>GAMGSDEQPHIGNYRLLKTLGKGNFAKVKRARHILTGREVAIKIIDKTQLNPTSLQKLFREVRIMKILNHPNIIKLFEVIETEKTLYLIMEYASKGEVYDYLVEHGRMKEKEARSKFRQIVSAVQYCHQKRIVHRDLKAENLLLDADMNIKIADFGFSNEFTVGGKLDTFCGSPPYAAPELFQGKKYDGPEVDVWSLGVILYTLVSGSLPFDGQNLKELRERVLRGKYRIPFYMSTD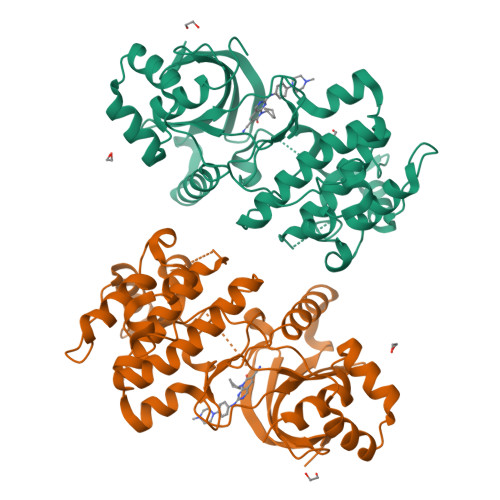CENLLKRFLVLNPIKRGTLEQIMKDRWINAGHEEDELKPFVEPELDISDQKRIDIMVGMGYSQEEIQESLSKMKYDEITATYLLLGRKSSE[2x]> GSMQRASRLKRELHMLATEPPPGITCWQDKDQMDDLRAQILGGANTPYEKGVFKLEVIIPERYPFEPPQIRFLTPIYHPNIDSAGRICLDVLKLPPKGAWRPSLNIATVLTSIQLLMSEPNPDDPLMADISSEFKYNKPAFLKNARQWTEKHAR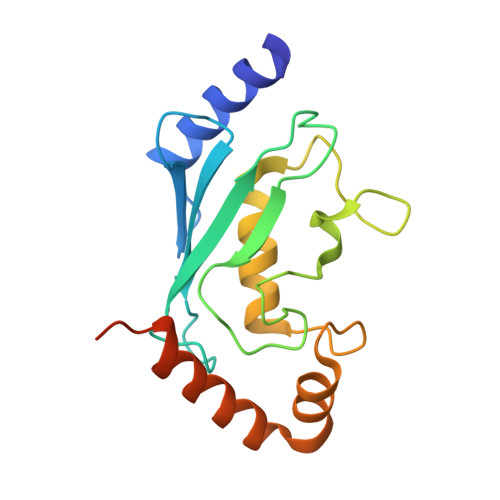QKQKADEEEMLDNLP7-[(3-CHLOROBENZYL)OXY]-4-[(METHYLAMINO)METHYL]-2H-CHROMEN-2-ONE 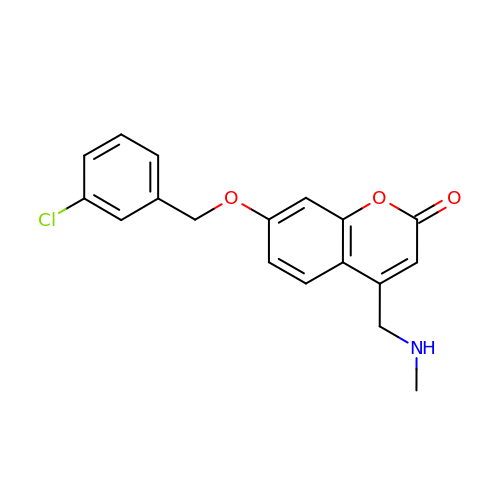| C18 H16 Cl N O3 | JMGUSOLCNQVZCT-UHFFFAOYSA-N> AMMNAFKEI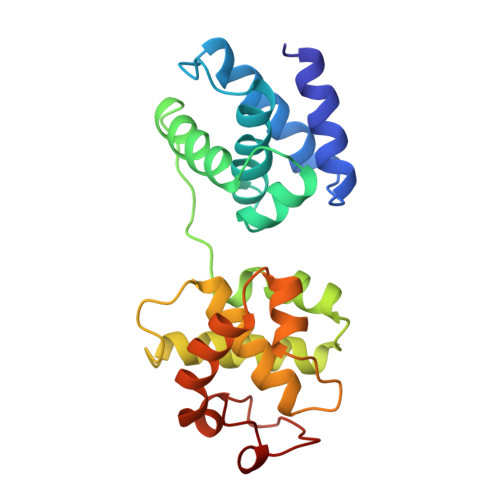TTMADRINLPRNKVDRTNNLFRQAYEQKSLKGRANDAIASACLYIACRQEGVPRTFKEICAVSRISKKEIGRCFKLILKALETSVDLITTGDFMSRFCSNLCLPKQVQMAATHIARKAVELDLVPGRSPISVAAAAIYMASQASAEKRTQKEIGDIAGVADVTIRQSYRLIYPRAPDLFPTDFKFDTPVDKLPQL To address this challenge, we develop a computational “anchor extension” methodology for targeting protein interfaces by extending a peptide chain around a non-canonical amino acid residue anchor. To test our approach using a well characterized model system, we design cyclic peptides that inhibit histone deacetylases 2 and 6 (HDAC2 and HDAC6) with enhanced potency compared to the original anchor (IC50 values of 9.1 and 4.4 nM for the best binders compared to 5.4 and 0.6 µM for the anchor, respectively). SHA can coordinate to the zinc ion in the active site of HDACs. In all the crystal structures we obtained, the thiol functional group of SHA coordinates the catalytic Zn2+ ion with a Zn2+– S separation of 2.3 Å in a distorted tetrahedral geometry reminiscent of that observed for the inhibitor Largazole.

To circumvent this problem, in design round 2, we built up macrocyclic scaffolds de novo inside the protein pocket to increase shape complementarity between the peptide and the HDAC2 pocket, and to make additional favorable interactions between the peptide backbone atoms and HDAC2. We also incorporated a Trp residue as an additional anchor that lays flat on a hydrophobic surface close to the active site, and mimics an aromatic ring observed in the same position in several small molecule inhibitors of HDACs. The macrocycle chain was extended from the SHA-Trp dimer, and the conformational space of closed macrocycles harboring these two residues was explored using generalized kinematic loop closure. The best tested peptide, des2.1.0 had an IC50 value of 49.3 nM, a four-fold improvement over method 1. To improve the affinity of des2.1.0, we mutated a D-Lys7 residue adjacent to a hydrophobic pocket in des2.1.0 to D-Met. The new des2.1.1 had an improved IC50 value of 16 nM for HDAC2. The crystal structure of des2.1.1 matches the designed orientation for the two anchor residues, SHA and Trp, with the position of the water molecules retained. While the electron density map for SHA and Trp are well resolved and match the designed model, the rest of the molecule appears to be in a conformation different from the solution structure obtained by NMR and the designed model; however, the electron density is too weak or absent, and the thermal B-factors are too high, for those residues to enable a meaningful comparison. This flexibility is consistent with the observation of multiple states during conformational sampling.

>[3x]AAYSQGGGKKKVCYYYDGDIGNYYYGQGHPMKPHRIRMTHNLLLNYGLYRKMEIYRPHKATAEEMTKYHSDEYIKFLRSIRPDNMSEYSKQMQRFNVGEDCPVFDGLFEFCQLSTGGSVAGAVKLNRQQTDMAVNWAGGLHHAKKSEASGFCYVNDIVLAILELLKYHQRVLYIDIDIHHGDGVEEAFYTTDRVMTVSFHKYGEYFPGTGDLRDIGAGKGKYYAVNFPMRDGIDDESYGQIFKPIISKVMEMYQPSAVVLQCGADSLSGDRLGCFNLTVKGHAKCVEVVKTFNLPLLMLGGGGYTIRNVARCWTYETAVALDCEIPNELPYNDYFEYFGPDFKLHISPSNMTNQNTPEYMEKIKQRLFENLRMLPHAPGVQMQAI;>XWTDNSMDK[3x]> QNPQQLSANLWAAVRARGCQFLGPAMQEEALKLVLLALEDGSALSRKVLVLFVVQRLEP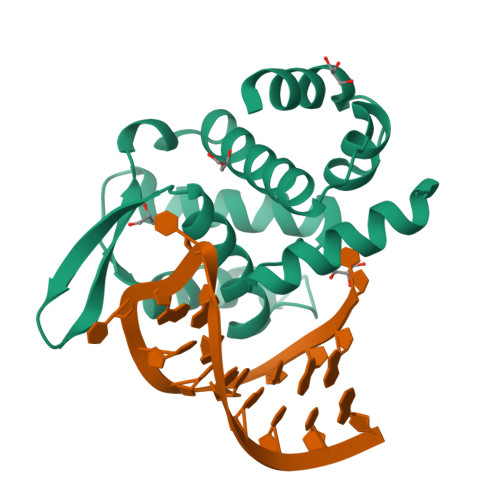RFPQASKTSIGHVVQLLYRASCFKVTKRDEDSSLMQLKEEFRSYEALRREHDAQIVHIAMEAGLRISPEQWSSLLYGDLAHKSHMQSIIDKLQSPE>[20x]GKKRPKPGGWNTGGSRYPGQGSPGGNRYPPQGGGTWGQPHGGGWGQPHGGGWGQPHGGGWGQPHGGGWGQGGGTHNQWNKPSKPKTNMKHMAGAAAAGAVVGGLGGYMLGSAMSRPMMHFG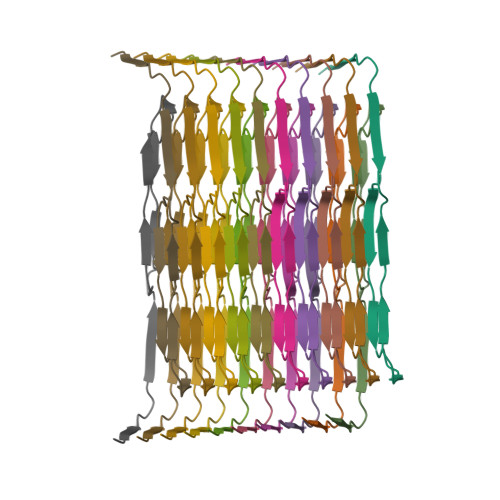ND N-ETHYLGUANIDINE 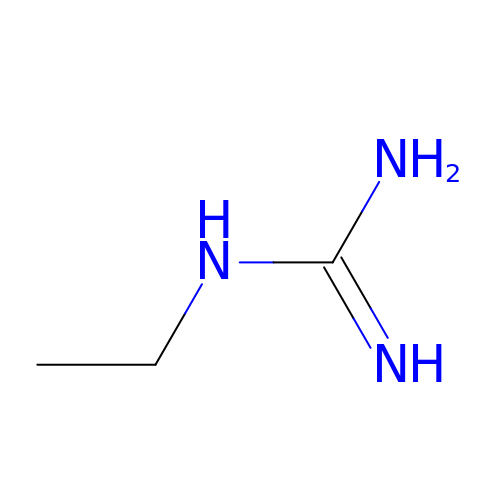| C3 H9 N3 | KEWLVUBYGUZFKX-UHFFFAOYSA-N>MPPNILSIFLHLLPILMFSSSCLGQGPPSPGYYPSSQITSLGFDQGYTNLWGPQHQRVDQG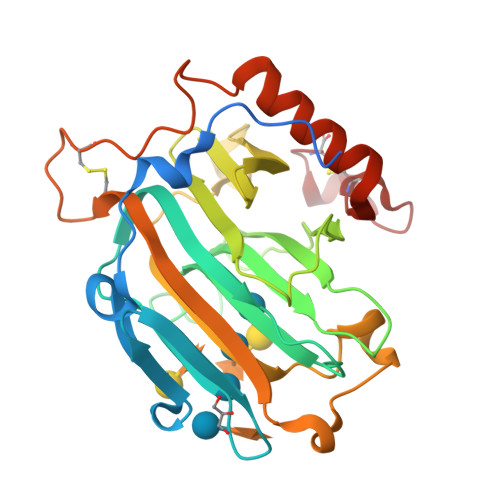SLTIWLDSTSGSGFKSINRYRSGYFGANIKLQSGYTAGVITSFYLSNNQDYPGKHDEIDIEFLGTIPGKPYTLQTNVFIEGSGDREMRIHLWFDPTQDYHNYAIYWTPSEIIFFVDDVPIRRYPRKSDATFPLRPLWVYGSVWDASSWATENGKYKADYRYQPFVGKYEDFKLGSCTVEAASSCNPASVSPYGQLSQQQVAAMEWVQKNYMVYNYCDDPTRDHTLTPEC[2x]5-[(4-chlorophenyl)methyl]-6-[[2-(dimethylamino)ethylamino]methyl]-4-oxidanyl-1~{H}-pyrimidine-2-thione 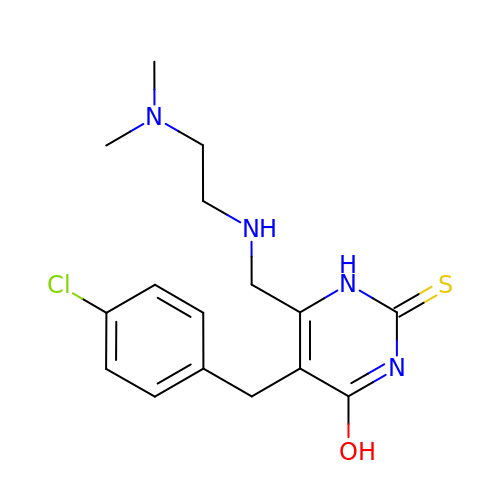| C16 H21 Cl N4 O S | BODROOXVZKSZLI-UHFFFAOYSA-N> VPACTVSNTTVDWQDVEIQTLSQNGNHEKEFTVNMRCPYNLGTMKVTITATNTYNNAILVQNTSNTSSDGLLVYLYNSNAGNIGTAITLGTPFTPGKITGNNADKTISLHAKLGYKGNMQNL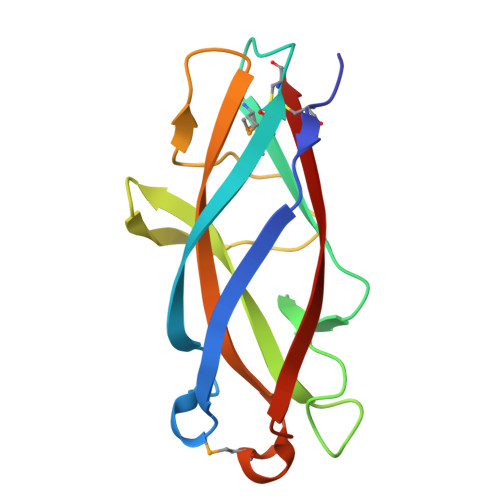IAGPFSATATLVASYS> GAACNVLFINSVEMESLTGPQAISKAVAETLVADPTPTATIVHFKVSAQG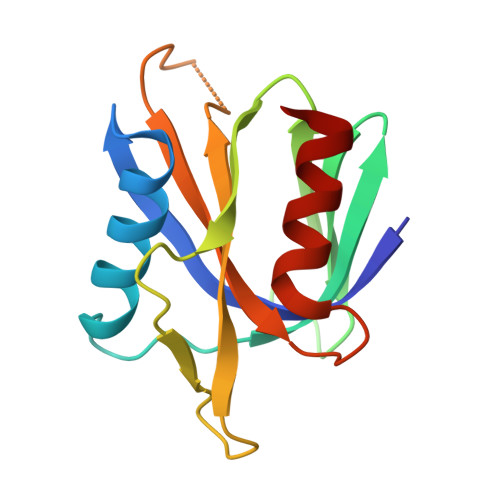ITLTDNQRKLFFRRHYPLNTVTFCDLDPQERKWTKTDGSGPAKLFGFVARKQGSTTDNVCHLFAELDPDQPAAAIVNFVSRVML> MLRYTCHALFLGSLVLLSGCDNSSSSSTSGSPGSPGNPGNPGTPGTPDPQDVVVRLPDVAVPGEAVQASARQAVIHLVDIAGITSSTPADYATKNLYLWNNETCDALSAPVADWNDVSTTPTGSDKYGPYWVIPLTKESGCINVIVRDGTNKLIDSDLRVSFSDFTDRTVSVIAGNSAVYDSRADAFRAAFGVALADAHWVDKTTLLWPGGENKPIVRLYYSHSSKVAADSNGEFSDKYVKLTPTTVNQQVSMRFPHLASYPAFKLPDDVNVDELLQGETVAIAAESDGILSSATQVQTAGVLDDTYAAAAEALSYGAQLTDSGVTFRVWAPTAQQVELVIYSADKKVIASHPMTRDSASGAWSWQGGSDLKGAFYRYAMTVYHPQSRKVEQYEVTDPYAHSLSTNSEYSQVVDLNDSALKPEGWDGLTMPHAQKTKADLAKMTIHESHIRDLSAWDQTVPAELRGKYLALTAQESNMVQHLKQLSASGVTHIELLPVFDLATVNEFSDKVADIQQPFSRLCEVNSAVKSSEFAGYCDSGSTVEEVLTQLKQNDSKDNPQVQALNTLVAQTDSYNWGYDPFHYTVPEGSYATDPEGTARIKEFRTMIQAIKQDLGMNVIMDVVYNHTNAAGPTDRTSVLDKIVPWYYQRLNETTGSVESATCCSDSAPEHRMFAKLIADSLAVWTTDYKIDGFRFDLMLYHPKAQILSAWERIKALNPDIYFFGEGWDSNQSDRFEIASQINLKGTGIGTFSDRLRDAVRGGGPFDSGDALRQNQGVGSGAGVLPNELTTLSDDQARHLADLTRLGMAGNLADFVLIDKDGAVKRGSEIDYNGAPGGYAADPTEVV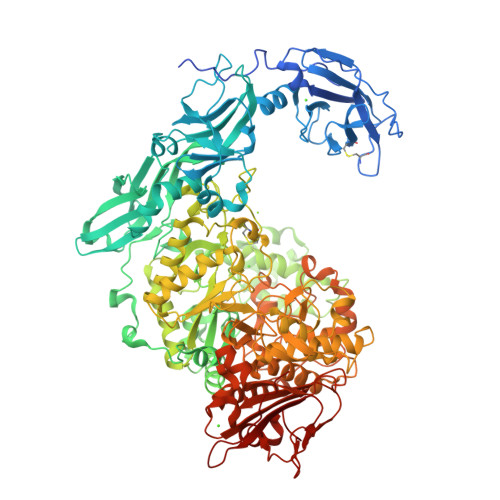NYVSKHDNQTLWDMISYKAAQEADLDTRVRMQAVSLATVMLGQGIAFDQQGSELLRSKSFTRDSYDSGDWFNRVDYSLQDNNYNVGMPRSSDDGSNYDIIARVKDAVATPGETELKQMTAFYQELTALRKSSPLFTLGDGATVMKRVDFRNTGADQQTGLLVMTIDDGMQAGASLDSRVDGIVVAINAAPESRTLQDFAGTSLQLSAIQQAAGDRSLASGVQVAADGSVTLPAWSVAVLELPQGESQGAGLPVSSK> GSSRAMGNEVAGVEDISVEITPSSKRNSDARRTSRNVCSNEERKRRKYFHMLYLVCLMVHGFIRNEWINSKRLSRKLSNLVPEKVFELLHPQKDEELPLRSTRKLLDGLKKCMELWQKHWKITKKYDNEGLYMRTWKEIEMSANNKRKFKTLKRSDFLRAVSKGHGDPDISVQGFVAMLRACNVNARLIMSCQPPDFTNMKIDTSLNGNNAYKDMVKYPIFWCEVWDKFSKKWITVDPVNLKTIEQVRLHSKLAPKGVACCERNMLRYVIAYDRKYGCRDVTRRYAQWMNSKVRKRRITKDDFGEKWFRKVITALHHRKRTKIDDYEDQYFFRRDESEGIPDSVQDLKNHPYYVLEQDIKQTQIVKPGCKECGYLKVHGKVGKVLKVYAKRDIADLKSARQWYMNGRILKTGSRCKKVIKRTVGRPKGEAEEEDERLYSFEDTELYIPPLASASGEITKNTFGNIEVFAPTMIPGNCCLVENPVAIKAARFLGVEFAPAVTSFKFERGSTVKPVLSGIVVAKWLREAIETAIDGIEFI;> GSGNASSGALGTTGGATDAAQGGPPGSIGLTVEDLLSLRQVVSGNPEALAPLLENISARYPQ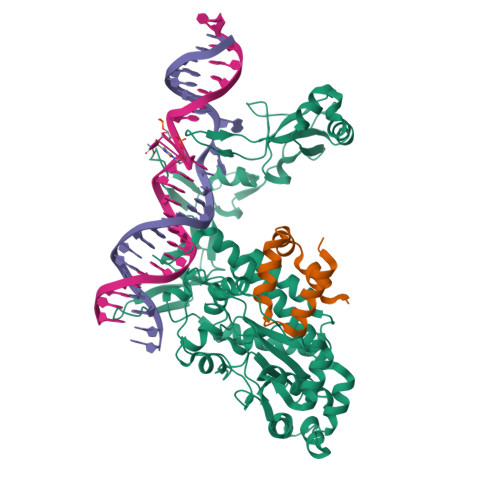LREHIMANPEVFVSMLLEAVGDNMQDVMEGADDMVEGEDIEVTGEAAAAGLGQGEGEGSFQVDYTPEDDQAISRLCELGFERDLVIQVYFACDKNEEAAANILFSDHAD4-(5-nitro-1H-indol-1-yl)phenyl alpha-D-mannopyranoside | C20 H20 N2 O8 | 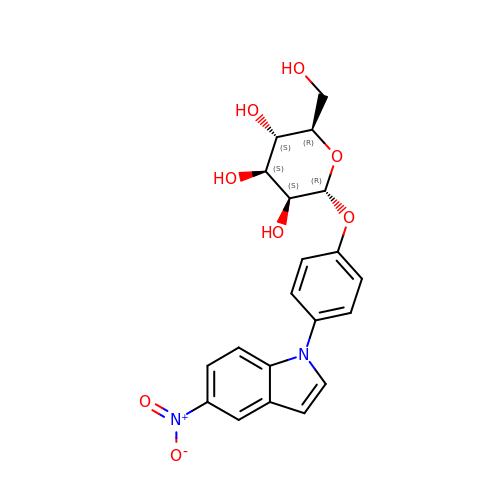CPRVANUZGRDTIH-SLHNCBLASA-N> MDAYSTRPLTLSHGSLEHVLLVPTASFFIASQLQEQFNKILPEPTEGFAADDEPTTPAELVGKFLGYVSSLVEPSKVGQFDQVLNLCLTEFENCYLEGNDIHALAAKLLQENDTTLVKTKELIKNYITARIMAKRPFDKKSNSALFRAVGEGNAQLVAIFGGQGNTDDYFEELRDLYQTYHVLVGDLIKFSAETLSELIRTTLDAEKVFTQGLNILEWLENPSNTPDKDYLLSI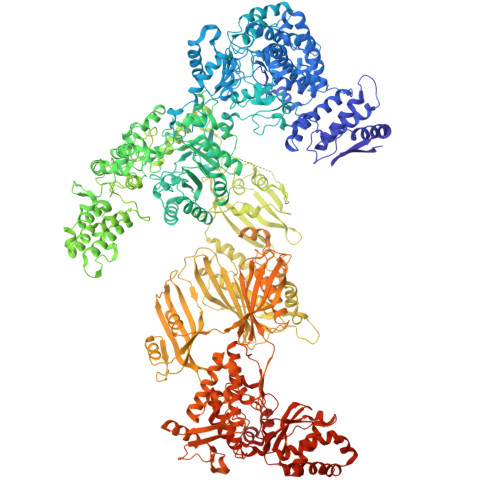PISCPLIGVIQLAHYVVTAKLLGFTPGELRSYLKGATGHSQGLVTAVAIAETDSWESFFVSVRKAITVLFFIGVRCYEAYPNTSLPPSILEDSLENNEGVPSPMLSISNLTQEQVQDYVNKTNSHLPAGKQVEISLVNGAKNLVVSGPPQSLYGLNLTLRKAKAPSGLDQSRIPFSERKLKFSNRFLPVASPFHSHLLVPASDLINKDLVKNNVSFNAKDIQIPVYDTFDGSDLRVLSGSISERIVDCIIRLPVKWETTTQFKATHILDFGPGGASGLGVLTHRNKDGTGVRVIVAGTLDINPDDDYGFKQEIFDVTSNGLKKNPNWLEEYHPKLIKNKSGKIFVETKFSKLIGRPPLLVPGMTPCTVSPDFVAATTNAGYTIELAGGGYFSAAGMTAAIDSVVSQIEKGSTFGINLIYVNPFMLQWGIPLIKELRSKGYPIQFLTIGAGVPSLEVASEYIETLGLKYLGLKPGSIDAISQVINIAKAHPNFPIALQWTGGRGGGHHSFEDAHTPMLQMYSKIRRHPNIMLIFGSGFGSADDTYPYLTGEWSTKFDYPPMPFDGFLFGSRVMIAKEVKTSPDAKKCIAACTGVPDDKWEQTYKKPTGGIVTVRSEMGEPIHKIATRGVMLWKEFDETIFNLPKNKLVPTLEAKRDYIISRLNADFQKPWFATVNGQARDLATMTYEEVAKRLVELMFIRSTNSWFDVTWRTFTGDFLRRVEERFTKSKTLSLIQSYSLLDKPDEAIEKVFNAYPAAREQFLNAQDIDHFLSMCQNPMQKPVPFVPVLDRRFEIFFKKDSLWQSEHLEAVVDQDVQRTCILHGPVAAQFTKVIDEPIKSIMDGIHDGHIKKLLHQYYGDDESKIPAVEYFGGESPVDVQSQVDSSSVSEDSAVFKATSSTDEESWFKALAGSEINWRHASFLCSFITQDKMFVSNPIRKVFKPSQGMVVEISNGNTSSKTVVTLSEPVQGELKPTVILKLLKENIIQMEMIENRTMDGKPVSLPLLYNFNPDNGFAPISEVMEDRNQRIKEMYWKLWIDEPFNLDFDPRDVIKGKDFEITAKEVYDFTHAVGNNCEDFVSRPDRTMLAPMDFAIVVGWRAIIKAIFPNTVDGDLLKLVHLSNGYKMIPGAKPLQVGDVVSTTAVIESVVNQPTGKIVDVVGTLSRNGKPVMEVTSSFFYRGNYTDFENTFQKTVEPVYQMHIKTSKDIAVLRSKEWFQLDDEDFDLLNKTLTFETETEVTFKNANIFSSVKCFGPIKVELPTKETVEIGIVDYEAGASHGNPVVDFLKRNGSTLEQKVNLENPIPIAVLDSYTPSTNEPYARVSGDLNPIHVSRHFASYANLPGTITHGMFSSASVRALIENWAADSVSSRVRGYTCQFVDMVLPNTALKTSIQHVGMINGRKLIKFETRNEDDVVVLTGEAEIEQPVTTFVFTGQGSQEQGMGMDLYKTSKAAQDVWNRADNHFKDTYGFSILDIVINNPVNLTIHFGGEKGKRIRENYSAMIFETIVDGKLKTEKIFKEINEHSTSYTFRSEKGLLSATQFTQPALTLMEKAAFEDLKSKGLIPADATFAGHSLGEYAALASLADVMSIESLVEVVFYRGMTMQVAVPRDELGRSNYGMIAINPGRVAASFSQEALQYVVERVGKRTGWLVEIVNYNVENQQYVAAGDLRALDTVTNVLNFIKLQKIDIIELQKSLSLEEVEGHLFEIIDEASKKSAVKPRPLKLERGFACIPLVGISVPFHSTYLMNGVKPFKSFLKKNIIKENVKVARLAGKYIPNLTAKPFQVTKEYFQDVYDLTGSEPIKEIIDNWEKYEQS> MDYKDDDDKALQSQASEEAKGPWQEADQEQQEPVGSPEPESEPEPEPEPEPVPVPPPEPQPEPQPLPDP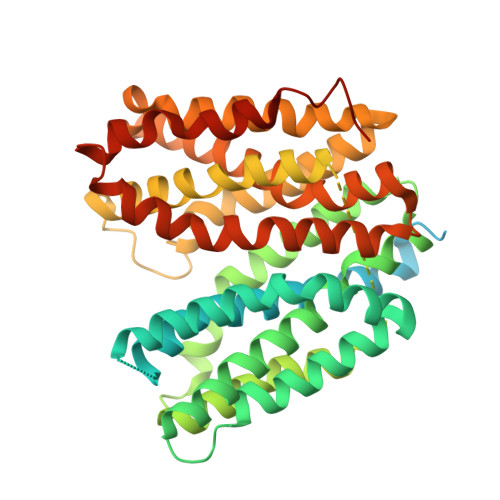APLPELEFESERVHEPEPTPTVETRGTARGFQPPEGGFGWVVVFAATWCNGSIFGIHNSVGILYSMLLEEEKEKNRQVEFQAAWVGALAMGMIFFCSPIVSIFTDRLGCRITATAGAAVAFIGLHTSSFTSSLSLRYFTYGILFGCGCSFAFQPSLVILGHYFQRRLGLANGVVSAGSSIFSMSFPFLIRMLGDKIKLAQTFQVLSTFMFVLMLLSLTYRPLLPSSQDTPSKRGVRTLHQRFLAQLRKYFNMRVFRQRTYRIWAFGIAAAALGYFVPYVHLMKYVEEEFSEIKETWVLLVCIGATSGLGRLVSGHISDSIPGLKKIYLQVLSFLLLGLMSMMIPLCRDFGGLIVVCLFLGLCNGFFITIMAPIAFELVGPMQASQAIGYLLGMMALPMIAGPPIAGLLRNCFGDYHVAFYFAGVPPIIGAVILFFVPSRLEEELRRRLTEPI RNA-binding proteins (RBPs) play critical roles in cell homeostasis by controlling gene expression post-transcriptionally. MSI2 is the dominant family member in the blood and is expressed in 70% of AML patients. It correlates with a poor clinical prognosis in multiple hematological malignancies.

We obtained a high-resolution crystal structure of the MSI2 RRM1 which allowed us to utilize a newly developed computational molecular modeling algorithm and perform docking analysis. We performed docking analysis to identify a putative binding region. Based on Ro’s ability to compete for MSI-RNA complexes, we hypothesized that the binding site is likely to be shared with the RNA binding site. Thus, we predicted a stacking interaction with F66 and R100 with Ro. Also, the K22 side chain and the NH backbone group from F97 formed stabilizing H-bonds with the oxygens from the aldehyde in the C2 position in the pyrimidine ring and the aldehyde from the opposite ring. To directly test our docking model, we mutated the putative interacting residues (K22A, F66A, F97A and R100A) and determined their ability to bind to Ro. This resulted in significantly reduced binding (F97A KD 69.5 ± 14.7 μM, R100A KD 148 ± 65 μM, F66A and K22A KD > 200 μM compared with 10.5 ± 0.3 μM for WT). Importantly, the single mutations did not disrupt RNA binding to MSI2 whereas the triple mutant completely inhibited its activity (KD > 50 μM). To provide additional evidence for the docking model, we performed NMR chemical shift analysis of 15N-labeled RRM1 and observed three main regions with structural changes by titrating MSI2 with Ro: (1) K22 region (with M21, I25, G26 and W30 shifts), (2) F66 region (with S61, G65, F66, and V67 shifts) and (3) F97 region (showing V95, A96, F97, and R100 shifts).

>MKMFIGGLSWQTSPDSLRDYFSKFGEIRECMVMRDPTTKRSRGFGFVTFADPASVDKVLGQPHHELDSKTIDPKVAFPRRAQPK[2x]> MASTNLDAVSVEIKVAGKVCDYVTMELFQSVSTHHRFKIKVNYRPDKPSVWAIGPDVIFKQLGEKVSIIMTHHESGEKTEFHGLISDIHVEGFDGNQGF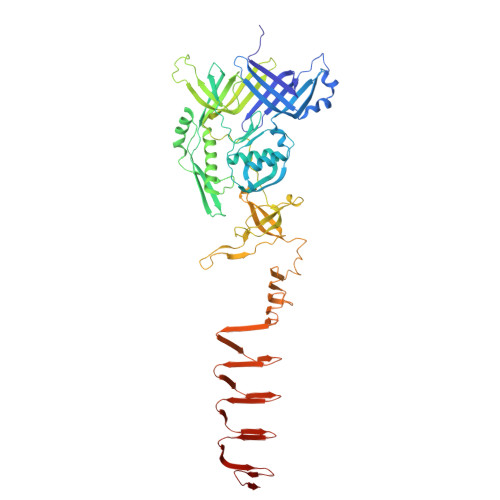VILEGGSPTILLDRDPAMDCYVEQNLNTIVSDILDKSGVKMNVTNNPKHTDIIPYVARYKETSYGFLSRLLRSYGEWFYYNGETLQIGDPEIDTESRAGYDVDLTGVSINATIRSLNHSTYEFDPVNDKFYYDYSGTPKGATLGSRSAEKCSEPIFPTEAKLPSIRPAYSAMDLEHYGDAGFHRNYSQLSQIKASSRYCGIRLGELVVTRVPESFPGVKITDLGRYRITEITHTVNYKGQYSNTFCGVPGGTPIMPWGDAVMPVAYPEMARVVSNDDPKNQGRVKVQFMWQEVDGGESYWMRVQSPDAGKSEQVAKNRGFVFIPEPGDLVMVGFEQGNPDRPYVTGSLFYKANSEGAATDNTVKSMRTRSGHTLEFKDDEGGDWGITLRDINGNVIHLNSKDKNIDITAPETITLTAKNVCINTEENVQITAKKNIDMTVEADINSSAKGNLLLQADKDVLTAAKGNVGIEAKSDINMVGKNIAVEGNSKITLNGGQTQVAGQQTTIQGAANKIEIM> NSTAELEELLMQRSLTDPQLQAAAAAAADFRILPDATVIKI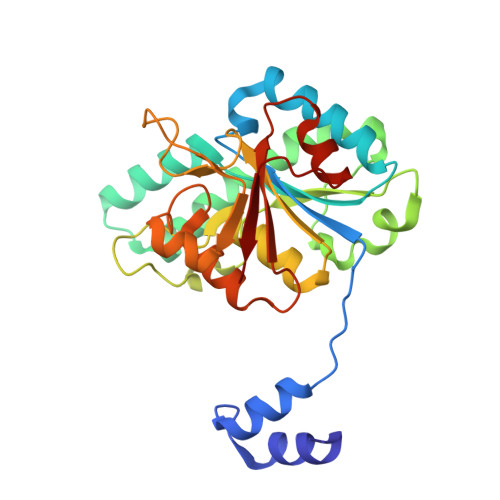GGQSVIDRGRAAVYPLVDEIVAARKNHKLLIGTGAGTRARHLYSIAAGLGLPAGVLAQLGSSVADQNAAMLGQLLAKHGIPVVGGAGLSAVPLSLAEVNAVVFSGMPPYKLWMRPAAEGVIPPYRTDAGCFLLAEQFGCKQMIFVKDEDGLYTANPKTSKDATFIPRISVDEMKAKGLHDSILEFPVLDLLQSAQHVREVQVVNGLVPGNLTRALAGEHVGTIITAS>[2x]MGMTQGAVKTTGKRSRAVSAKKKAILSAALDTFSQFGFHGTRLEQIAELAGVSKTNLLYYFPSKEALYIAVLRQILDIWLAPLKAFREDFAPLAAIKEYI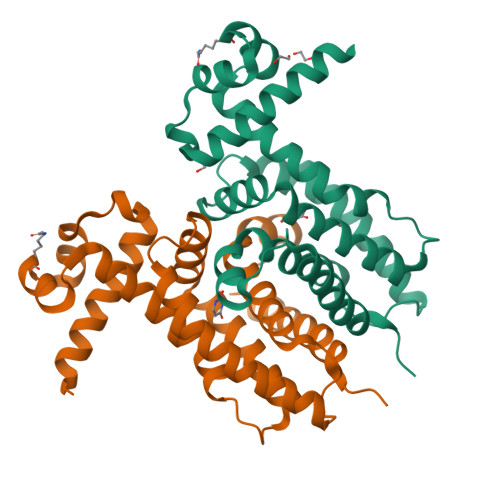RLKLEVSRDYPQASRLFCMEMLAGAPLLMDELTGDLKALIDEKSALIAGWVKSGKLAPIDPQHLIFMIWASTQHYADFAPQVEAVTGATLRDEVFFNQTVENVQRIIIEGIRPRHHHHHH2-[2-(3-CHLORO-PHENYL)-2-HYDROXY-ACETYLAMINO]-N-[4-GUANIDINO-1-(THIAZOLE-2-CARBONYL)-BUTYL]-3-METHYL-BUTYRAMIDE | 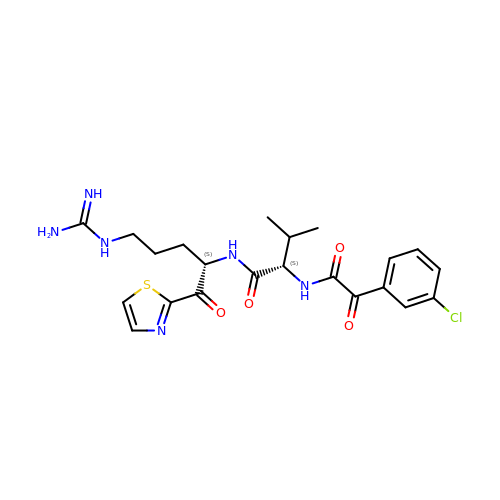C22 H27 Cl N6 O4 S | NZMZDRVEUJTADA-HOTGVXAUSA-N> SNAERKYSTFYEQRATLFEELPVTSKDIIFLGNSITNGCEWAELFQNKNVKNRGI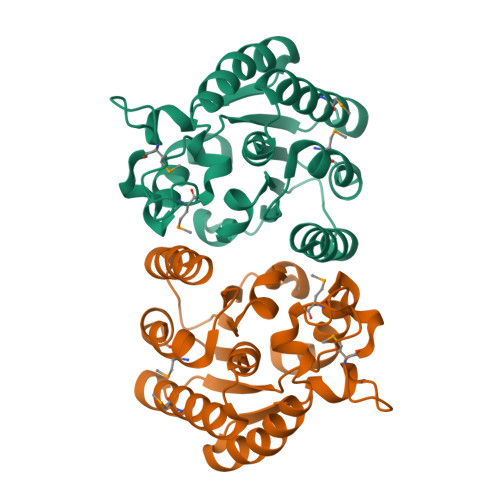SGDICMGVYDRLDPIVKGKPAKIFLLIGINDVSRGTSADKIISEISMIVRKIKQESPKTKLYLQSVLPVNDCYGMFNGHTSRWQVVKQINDLLEPLAVKEGVAYIDLYSHFVEKETGKMNPVYTNDGLHLLGKGYLLWRDIVKPYVD> MDTSKLKPNDPRVKYETKQIRGKTYSYILGEPAGPKLETVVLVHGWPDMAFGWRHQIPYLMSLGFQVVAPNMLGYAGTDAPRDLSQFTLKSVSADIAELARSFVGQDGQIVLGGHDWGGAVVWRTAYYHPELVKAVFSVCTPLHPLSAEYKPLEDIVAAGHMLNFKYQLQLKGPDVEARIQGKDMLRRFFRAMFGGRGPNGEAGFSTSDGVHFDVLDKIGAPPLLDEQELEYYVEQYALQEAPELRGPLNWYRTRELNAKDEMDRAKNGPPLRFEMPALFVAASKDNALPPAMSKGMDAFYKDLTRAEVDATHW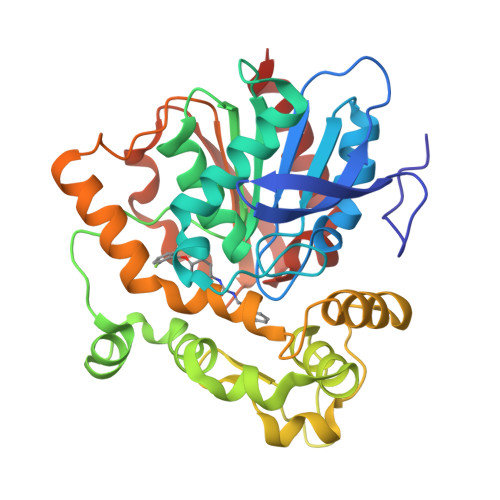ALTQAGDEVNRVIGEWLNKALG> GAEFMAVAGAVSGEPLVHWCTQQLRKTFGLDVSEEIIQYVLSIESAEEIREYVTDLLQGNEGKKGQFIEELITKWQKNDQELISDPLQQCFKKDEILDGQKSGDHLKRGRKKGRNRQEVPAFTEPDTTAEVKTPFDLAKAQENSNSVKKKTKFVNLYTREGQDRLAVLLPGRHPCDCLGQKHKLINNCLICGRIVCEQEGSGPCLFCGTLVCTHEEQDILQRDSNKSQKLLKKLMSGVENSGKVDISTKDLLPHQELRIKSGLEKAIKHKDKLLEFDRTSIRRTQVIDDESDYFASDSNQWLSKLERETLQKREEELRELRHASRLSKKVTIDFAGRKILEEENSLAEYHSRLDETIQAIANGTLNQPLTKLDRSSEEPLGVLVNPNMYQSPPQWVDHTGAASQKKAFRSSGFGLEFNSFQHQLRIQDQEFQEGFDGGWCLSVHQPWASLLVRGIKRVEGRSWYTPHRGRLWIAATAKKPSPQEVSELQATYRLLRGKDVEFPNDYPSGCLLGCVDLIDCLSQKQFKEQFPDISQESDSPFVFICKNPQEMVVKFPIKGNPKIWKLDSKIHQGAKKGLMKQNKAV;> GAEFHYPHVYDSQAEAMKTSAFIAGAKMILPEGIQRENNKLYEEVRIPYSEPMPLSFEEKPVYIQDLDEIGQLAFKGMKRLNRIQSIVFETAYNTNENMLICAPTGAGKTNIAMLTVLHEIRQHFQQGVIKKNEFKIVYVAPMKALAAEMTDYFSRRLEPLGIIVKELTGDMQLSKSEILRTQMLVTTPEKWDVVTRKSVGDVALSQIVRLLILDEVHLLHEDRGPVLESIVARTLRQVESTQSMIRILGLSATLPNYLDVATFLHVNPYIGLFFFDGRFRPVPLGQTFLGIKCANKMQQLNNMDEVCYENVLKQVKAGHQVMVFVHARNATVRTAMSLIERAKNCGHIPFFFPTQGHDYVLAEKQVQRSRNKQVRELFPDGFSIHHAGMLRQDRNLVENLFSNGHIKVLVCTATLAWGVNLPAHAVIIKGTQIYAAKRGSFVDLGILDVMQIFGRAGRPQFDKFGEGIIITTHDKLSHYLTLLTQRNPIESQFLESLADNLNAEIALGTVTNVEEAVKWISYTYLYVRMRANPLAYGISHKAYQIDPTLRKHREQLVIEVGRKLDKAQMIRFEERTGYFSSTDLGRTASHYYIKYNTIETFNELFDAHKTEGDIFAIVSKAEEFDQIKVREEEIEELDTLLSNFCELSTPGGVENSYGKINILLQTYISRGEMDSFSLISDSAYVAQNAARIVRALFEIALRKRWPTMTYRLLNLSKVIDKRLWGWASPLRQFSILPPHILTRLEEKKLTVDKLKDMRKDEIGHILHHVNIGLKVKQCVHQIPSVMMEASIQPITRTVLRVTLSIYADFTWNDQVHGTVGEPWWIWVEDPTNDHIYHSEYFLALKKQVISKEAQLLVFTIPIFEPLPSQYYIRAVSDRWLGAEAVCIINFQHLILPERHPPHTELLDLQPLPITALGCKAYEALYNFSHFNPVQTQIFHTLYHTDCNVLLGAPTGSGKTVAAELAIFRVFNKYPTSKAVYIAPLKALVRERMDDWKVRIEEKLGKKVIELTGDVTPDMKSIAKADLIVTTPEKWDGVSRSWQNRNYVQQVTILIIDEIHLLGEERGPVLEVIVSRTNFIS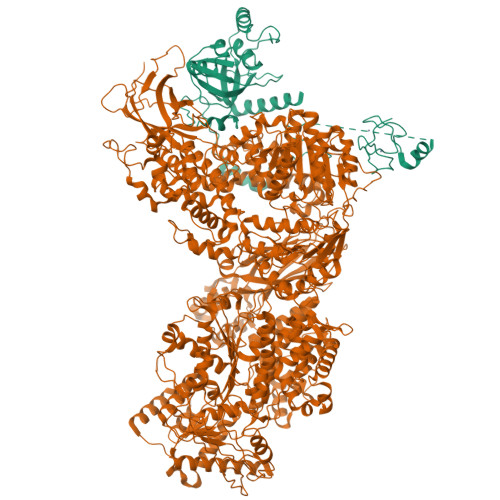SHTEKPVRIVGLSTALANARDLADWLNIKQMGLFNFRPSVRPVPLEVHIQGFPGQHYCPRMASMNKPAFQAIRSHSPAKPVLIFVSSRRQTRLTALELIAFLATEEDPKQWLNMDEREMENIIATVRDSNLKLTLAFGIGMHHAGLHERDRKTVEELFVNCKVQVLIATSTLAWGVNFPAHLVIIKGTEYYDGKTRRYVDFPITDVLQMMGRAGRPQFDDQGKAVILVHDIKKDFYKKFLYEPFPVESSLLGVLSDHLNAEIAGGTITSKQDALDYITWTYFFRRLIMNPSYYNLGDVSHDSVNKFLSHLIEKSLIELELSYCIEIGEDNRSIEPLTYGRIASYYYLKHQTVKMFKDRLKPECSTEELLSILSDAEEYTDLPVRHNEDHMNSELAKCLPIESNPHSFDSPHTKAHLLLQAHLSRAMLPCPDYDTDTKTVLDQALRVCQAMLDVAANQGWLVTVLNITNLIQMVIQGRWLKDSSLLTLPNIENHHLHLFKKWKPIMKGPHARGRTSIESLPELIHACGGKDHVFSSMVESELHAAKTKQAWNFLSHLPVINVGISVKGSWDDLVEGHNELSVSTLTADKRDDNKWIKLHADQEYVLQVSLQRVHFGFHKGKPESCAVTPRFPKSKDEGWFLILGEVDKRELIALKRVGYIRNHHVASLSFYTPEIPGRYIYTLYFMSDCYLGLDQQYDIYLNVTQASLSAQVNTKVSDSLTDLALK> MSLSTAADLLRQGAACSVLYLTSVETESLTGPQAVARASSAALSCSPRPTPAVVHFKVSAQGITLTDNQRKLFFRRHYPVNSITFSSTDPQDRRWTNPDGTTSKIFGFVAKKPGS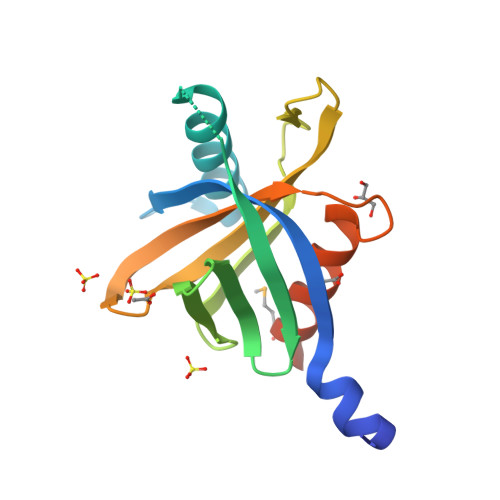PWENVCHLFAELDPDQPAGAIVTFITKVMLGQRKEGHHHHHH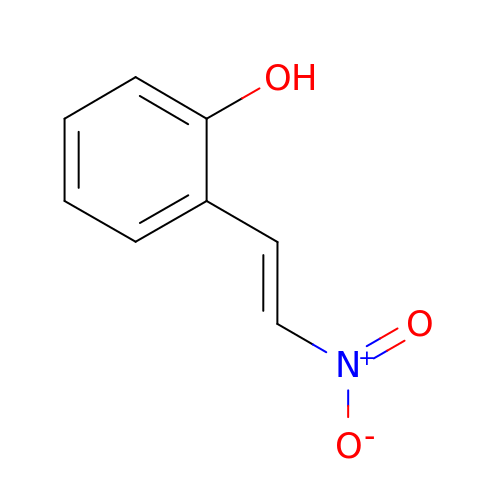2-[(E)-2-nitroethenyl]phenol | C8 H7 N O3 | PMDYAIGGZBRBFX-AATRIKPKSA-N> STIQPGTGYNNGYFYSYWNDGHGGVTYTNGPGGQFSVNWSNSGDFVGGKGWQPGTKNKVINFSGSYNPNGNSYLSVYGWSRNPLIEYYIVENFGTYNPSTGATKLGEVTSDGSVYDIYRTQRVNQPSIIGTATFYQYWSVRRNHRSSGSVNTANHFNAWAQQGLTLGTMDYQIVAVEG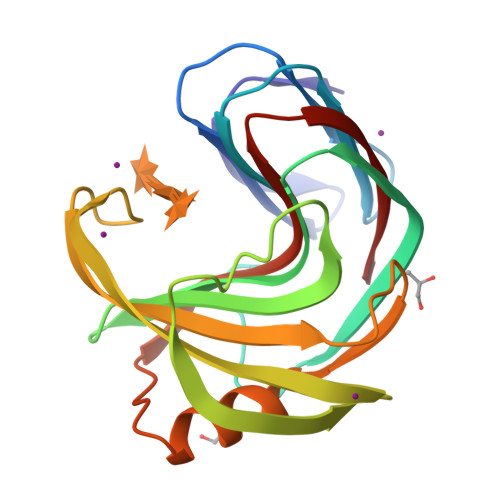YFSSGSASITVS> TGSLSFSFPKFAPNQPYLINQGDALVTSTGVLQLTNVVNGVPSSKSLGRALYAAPFQIWDSTTGNVASFVTSFTFIIQAPNPATTADGLAFFLAPVDTQPLDLGGMLGIFKDGYFNKSNQIVAVEFDTFSNGDWDPKGRHLGINVNSIESIKTVPWNWTNGEVANVFISYEASTKSLTASLVYPSLETSFIIDAIVDVKIVLPEW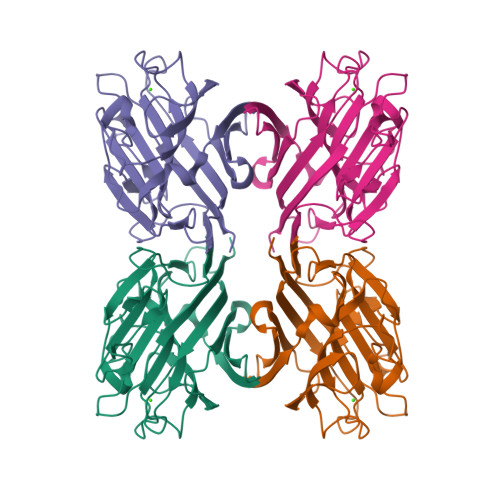VRFGFSATTGIDKGYVQTNDVLSWSFESNLPG2-(4-fluorophenyl)acetohydrazide | C8 H9 F N2 O | 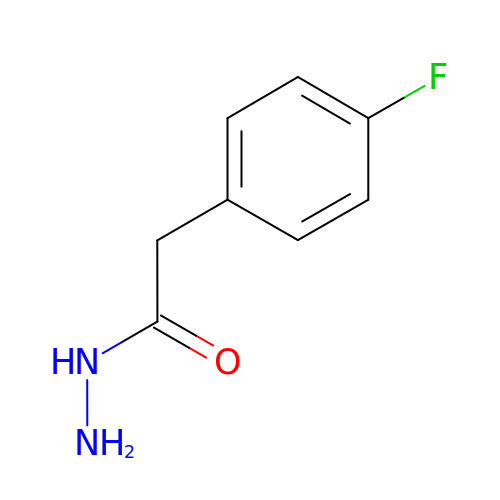PFBNINAURUGQRR-UHFFFAOYSA-N>GSMSRSKRDNNFYSVEIGDSTFTVLKRYQNLKPIGSGAQGIVCAAYDAILERNVAIKKLSRPFQNQTHAKRAYRELVLMKCVNHKNIIGLLNVFTPQKSLEEFQDVYIVMELMDANLCQVIQMELDHERMSYLLYQMLCGIKHLHSAGIIHRDLKPSNIVVKSDCTLKILDFGLARTAGTSFMMTPYVVTRYYRAPEVILGMGYKENVDIWSVGCIMGEMIKGGVLFPGTDHIDQWNKVIEQLGTPCPEFMKKLQPTVRTYVENRPKYAGYSFEKLFPD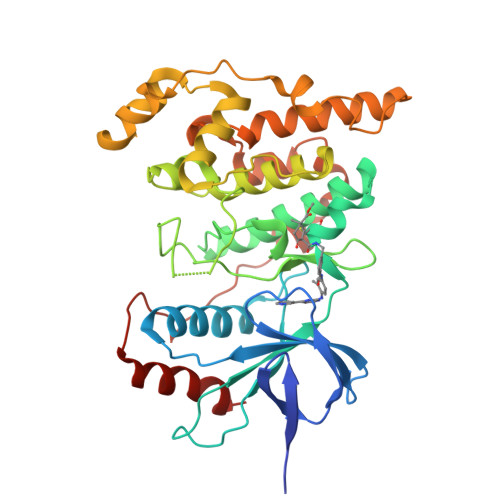VLFPADSEHNKLKASQARDLLSKMLVIDASKRISVDEALQHPYINVWYDPSEAEAPPPKIPDKQLDEREHTIEEWKELIYKEVMDLE[3x]>[4x]MKTINIVAGGPKNLIPDLTGYT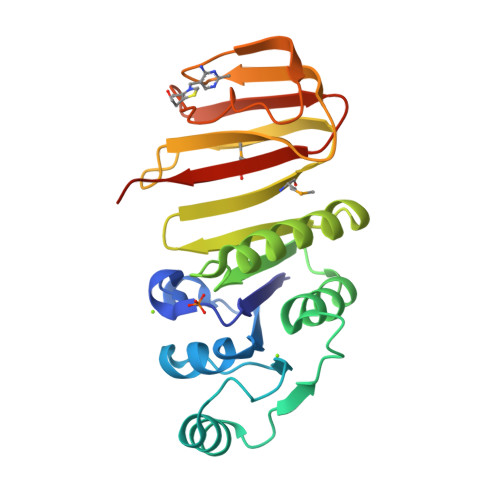DEHTLWIGVDKGTVTLLDAGIIPVEAFGDFDSITEQERRRIEKAAPALHVYQAEKDQTDLDLALDWALEKQPDIIQIFGITGGRADHFLGNIQLLYKGVKTNIKIRLIDKQNHIQMFPPGEYDIEKDENKRYISFIPFSEDIHELTLTGFKYPLNNCHITLGSTLCISNELIHSRGTFSFVKGILIMIRSTDLEHHHHHH> GSAMGMSNTQAERSIIGMIDMFHKYTGRD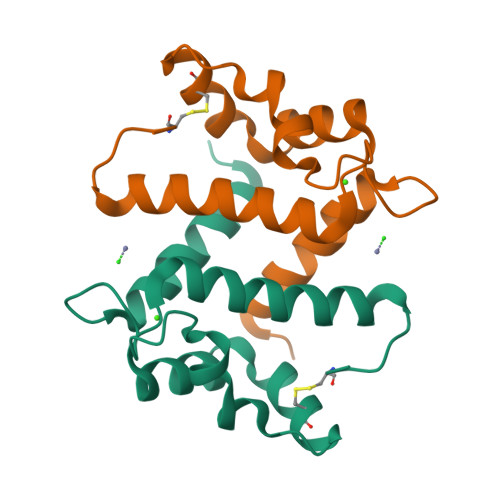GKIEKPSLLTMMKENFPNFLSACDKKGIHYLATVFEKKDKNEDKKIDFSEFLSLLGDIAADYHKQSHGAAPCSGGSQAAA Chromatin remodeling complex NoRC (nucleolar remodeling complex) interacts with the rDNA promoter regions of silent genes repressing rDNA transcription. It consists of TIP5 (TTF-I interacting protein 5), also known as BAZ2A (bromodomain [BRD] adjacent to zinc finger domain protein 2A), which is the largest subunit, and the adenosine triphosphatase (ATPase) SNF2h (sucrose nonfermenting protein 2 homologue). BAZ2B shares 29% sequence identity with TIP5 at the full-length level and harbors similar domain organization. Both proteins contain a MBD (methyl-CpG-binding domain), also known as TAM (TTF-IIP5, ARBP, MeCP1) domain, AT-hook DNA-binding domains, DDT (DNA binding homeobox and different transcription factors), and a PHD (plant homeodomain) zinc finger adjacent to a BRD at their C terminus. Our crystal structures combined with biophysical and mutagenesis data demonstrate that PHD zinc fingers recognize N-terminal unmodified H3K4 tail, whereas the TIP5 and BAZ2B BRDs recognize H4K16ac and H3K14ac, respectively, with specificity pattern KacXXR.

The crystal structures of free-state TIP5 BRD as well as in complex with H4K16acK20ac were solved at 1.76 and 1.65 Å resolution, respectively. The H4 peptide conformation extended from its N terminus at the ZA loop region to the C terminus at the BC loop region of the BRD. Several residues V1822, V1827, F1872, and V1879 provided a hydrophobic environment to accommodate the hydrophobic segment of the K16ac side chain orienting the N-acetyl group toward the amide nitrogen of N1873. Similar to the BAZ2B complex, further stabilizing contributions were provided by interaction with the conserved water network. Only few side-chain interactions with BRD residues were involved in the molecular interface, which was mediated mainly through the peptide backbone hydrogen bond interactions with TIP5 residues N1873, F1872, E1874, and R1832. An interesting interaction involved the guanidine group of H4R19 that oriented toward the BC loop, forming a hydrogen bond between its Nε-H and the carbonyl of Q1870, and a salt bridge with the two acidic residues E1874 and D1875. These features demonstrate a conservation of BRD-histone interactions between TIP5 and BAZ2B in this region. Analyses of our peptide arrays, ITC data, and crystal structure suggests that much of the recognition specificity for H4K16ac by the TIP5 BRD in vitro is due to the intricate network of interactions formed by the R19 side chain. ITC determined an affinity of 23 μM for H4K16ac (G14-A15-K16ac-R17-H18-R19-K20-V21-L22), whereas binding affinity decreased 2-fold for the H4K12acK16ac (G9-L10-G11-K12ac-G13-G14-A15-K16ac-R17). However, the NoRC BRDs are characterized by a more negative electrostatic potential in this region, favoring interaction with positively charged residues such as H4R19, thus offering a rationale for the weaker interaction of this peptide with BPTF.

>[2x]SMHSDLTFCEIILMEMESHDAAWPFLEPVNPRLVSGYRRIIKNPMDFSTMRERLLRGGYTSSEEFAADALLVFDNCQTFNEDDSEVGKAGHIMRRFFESRWEEFYQ;>[2x]GAKRHRKVL The rotating flagellar filament primarily functions as a propeller, acting as an Archimedean screw, and supercoiling of the filament is essential as rotations of a straight filament do not generate thrust. Here, we show the atomic cryo-electron microscopy structures for flagellar filaments from enterohemorrhagic Escherichia coli O157:H7, enteropathogenic E. coli O127:H6, Achromobacter, and Sinorhizobium meliloti, where the outer domains dimerize or tetramerize to form either a sheath or a screw-like surface. A shared feature in all four structures is the formation of symmetrical homodimers between the outer domains of flagellin subunits, with one outer domain rotated 180° relative to the other. These symmetrical dimers are the result of outer domains being able to adopt either an “up” or “down” conformation.

A 6.7 Å resolution volume was reconstructed asymmetrically where all flagellin subunits could be fitted into the density. Analysis of this low-resolution structure revealed the seam, which involves the lack of D2 dimer formation between two flagellin subunits. This seam is a consequence of a reduction of symmetry along the 9-start helices of a flagellar filament composed of dimeric flagellin such as EHEC H7. The two outer domain subunits in the seam still form Sn:Sn + 22 dimers in domain D4. However, rather than forming an Sn:Sn + 6 or Sn:Sn + 11 dimer in domain D2, the two-seam subunits form Sn:Sn + 5 dimers with each other similar to those forming the EHEC H7 and the Achromobacter ODSs. In the non-helical perturbation model, subunit pairing introduced a seam causing a discontinuity in the helical lattice, much as such a seam or discontinuity exists in microtubules.

>[2x]MAQVINTNSLSLITQNNINKNQSALSSSIERLSSGLRINSAKDDAAGQAIANRFTSNIKGLTQAARNANDGISVAQTTEGALSEINNNLQRIRELTVQASTGTNSDSDLDSIQDEIKSRLDEIDRVSGQTQFNGVNVLAKDGSMKIQVGANDGQTITIDLKKIDSDTLGLNGFNVNGKGETANTAATLKDMSGFTAAAAPGGTVGVTQYTDKSAVASSVDILNAVAGADGNKVTTSADVGFGTPAAAVTYTYNKDTNSYSAASDDISSANLAAFLNPQARDTTKATVTIGGKDQDVNIDKSGNLTAADDGAVLYMDATGNLTKNNAGGDTQATLAKVATATGAKAATIQTDKGTFTSDGTAFDGASMSIDANTFANAVKNDTYTATVGAKTYSVTTGSAAADTAYMSNGVLSDTPPTYYAQADGSITTTEDAAAGKLVYKGSDGKLTTDTTSKAESTSDPLAALDDAISQIDKFRSSLGAVQNRLDSAVTNLNNTTTNLSEAQSRIQDADYATEVSNMSKAQIIQQAGNSVLAKANQVPQQVLSLLQG>[8x]GSEELLDLFNRQVTQEFTASQVYLSASIWFDQNDWEGMAAYMLAQSAEEREHGLGFVDFANKRNIPIELQAVPAPVSCAEWSSPEDVW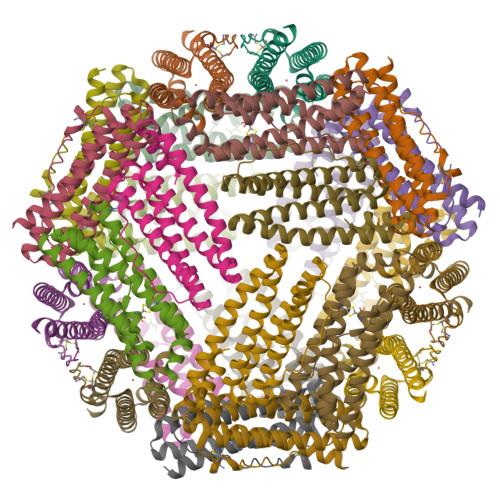QSILELEQANTRSLLNLAEAASTCHDFAVMAFLNPFHLQQVNEEDKIGSILAKVTDENRTPGLLRSLDVVSFLGPCLFRSV Therefore, the β-xylosidase catalyzing the removal of xylosyl from XDT would play a prominent role in reducing both of the resource waste and pollution to environment. Here we present the crystal structures of LXYL-P1-2 and its complex with XDT. Each monomer comprises three domains as some GH3 members. Sequence alignment of LXYL-P1-2 indicates that Asp300 and Glu529 might act as the catalytic nucleophile and the acid/base residues, respectively.

To improve formation of good quality crystals, LXYL-P1-2 was endoglycosidase-treated before crystallization. The first 43 residues were missing in the electron density map, partially supporting the existence of the KEX27 cleavage site (Ile32Phe33Arg34Arg35). The structure of the four monomers are essentially same without any remarkable difference. Domain 3 (residue 664–803) is connected to domain 2 by linker 2 (residue 601–663) and has a fibronectin type III (FnIII) fold. Seven Asn residues (81, 272, 342, 385, 457, 576, and 635) are found to link with different types of oligosaccharide even after treated by endoglycosidase H. In LXYL-P1-2 structure, the distance of these two residues is 5.5 Å, consistent with the proposed retaining catalytic mechanism in GH3 family. In the substrate free enzyme, Glu529 forms hydrogen bond to the side-chain of Arg218 and the main-chain NH of Ser466. The catalytic pocket of each monomer faces to the outside of tetramer. The tetramer formation seems not influence on the active pocket, but contributes to the highly thermal stability of LXYL-P1-2. Two interfaces are defined in the LXYL-P1-2 tetramer. The interface B was never reported in GH3 family.

>MFPARLSLAVLFSVSPALAYFSGLGLGSERSIFRRDLNSTGDESNSTQWPAPLANGGKSWASAFKKAKATVTEMTVEELANITSGVIGLCSGVTGAVTRLGIPEFCLQDGPIGPRGVHGSSQFPAGLTVAATWDRTLMYARARGMGQEFHDQGVHLALAPVTGGPLGRTPLNGRGWEGTFADPYACGEASYLSVKGLTDAGVATVSKHWIAYEQETSRNLYIDIDGVSQADIQLPISSNVDDLTMHELYMWSFAEAVRAGTNHIMCSYNRINNTHSCSNAKGLNQLLKTELNFQGGVVSDWGGQWDSVPAAENGLDVAMPGKGFLGALGDFWGATLVELINNGTVSEDLVRDKAVRILTGYYYLGQDTNPPPPFVYNTIGAPTLNATSGYRNVRKPGTAELIKEIGSASVTLLKNTGSLPLKHPQRIAVLGNDATYNVLGPNACGLANSACDIDNLNGTLTTGGGSGSALSPYTITPLEALQKRAIEDNAEIAAVVANSNTTTGAEDAIAALLPDADVTFVFLNRYSEEGADAPDFSLGGDGDNLMDLAVTYSSNVVVVIHTTGVVDIEKWADNPNVTAILVAYLPGQEAGNSLVPVLYGDVAPSGKLPWTWGKSIDDYVPNGVVYTDAYSPQSNFTEGVFIDYRWFDKMGITPRYEFGFGLSYTTFTYSNLIVDHGRWAKDYSSVMETAEPFAEWDGTNSLYDVIFTVFATITNTGNLTGSEVAQLYISIPGDNQPVRQLRGFDKIKDLPVGDSAVVTFPIRRKDVSSWSVVDQLWYVPNGDFLISVGGSSRDLPLNTTWTPHHHHHH[4x]> MLEAKFEEASLFKRIIDGFKDCVQLVNFQCKEDGIIAQAVDDSRVLLVSLEIGVEAFQEYRCDHPVTLGMDLTSLSKILRCGNNTDTLTLIADNTPDSIILLFEDTKKDRIAEYSLKLMDIDADFLKIEELQYDSTLSLPSSEFSKIVRDLSQLSDSINIMITKETIKFVADGDIGSGSVIIKPFVDMEHPETSIKLEMDQPVDLTFGAKYLLDIIKGSSLSDRVGIRLSSEAP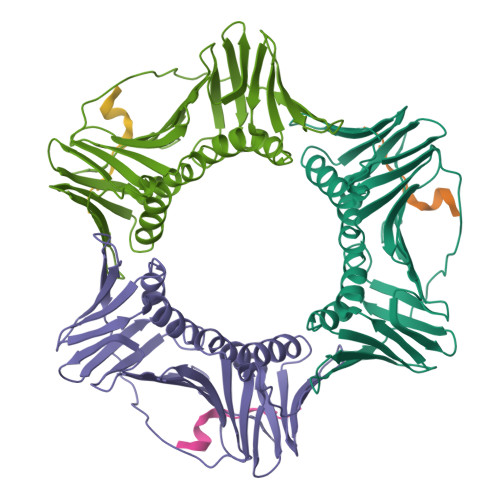ALFQFDLKSGFLQFFLAPKFNDEE;> AGKKPKQATLARFFTSMKNKPT>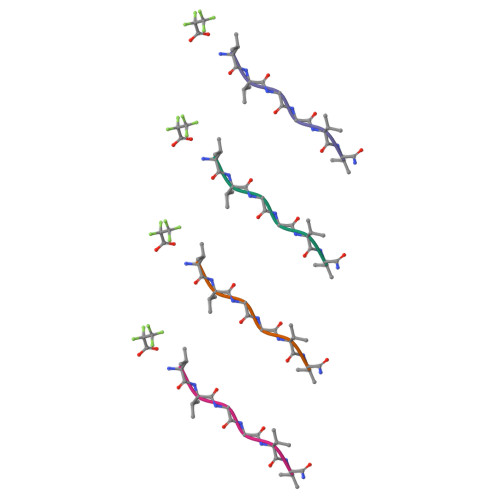 VVGGVVX> MGIKGIYKEIGSGERISLCKLAIDHLEQHNRPLRLAIDMAIWQFQIQAARGGSNPAIRTLFYRFVRLLSLGIHPIFVFDGPNKPIFKRNRRSGTGNGVSTAMAKRLIRLFGFTAHDAPGEAEAECAYLEQQGIVDAVLSEDVDTIMFGSRVTLRDWSSEGSKGGPPTHVTLHDAKKIAEGPSGLDREGMVLVALMSGGDYLPDGIPGCGIKVACQAAKAGFGKELCRIKRADKEAITEW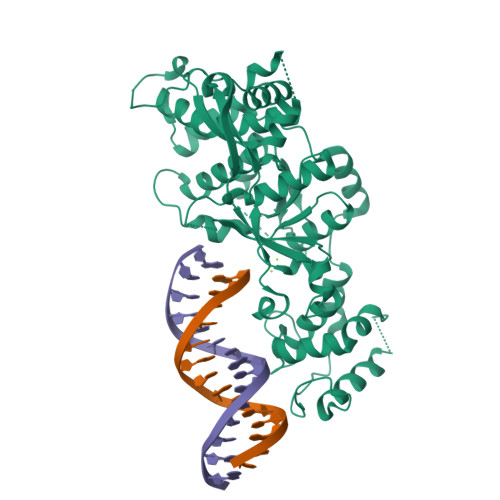KQRLLHELRTNESGFFRTKHKALEIPENFPNMEVLRYYTHPVVSSPATIERLRQEFPPSSTVDIAGLREFTRETFDWTFRPGAIKLIKVLAPGLLVQRCLDRYVSGPRIDDPDLKKKEESTLVKGISMRREHFSTDATPELRVSFIPAELVGLDPGQEPEVQVEAFGRSGLALNSDDEFDEDISSSQKAPKKPFDPWQPDLAWVPETILKLGVPVTVEDWEEGQRSKGRAKEDKTAAKAKRKTKIIQSNMPAGALDKYVTVTKNISDTTVKSKESAPITIPSSPPKPSSQP>[6x]GMSAGQSSLSFAHGDETHPIEQKAFIGVDSAAGNVVKQFHAALQMGNEAIVRQSLAANVQIYEGGKVERSLTEYANHHMLADMAYLK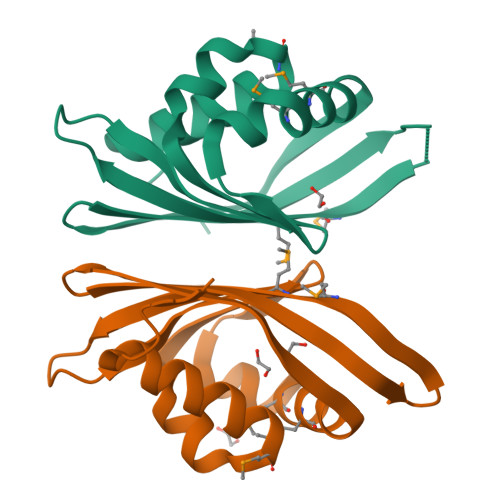GLTITPKEHQITITGDIAISTSISHAQGEYKGKSIDSMTMETLVLIKQADGRWKITHVHWS Flavin-dependent halogenases regioselectively introduce halide substituents into electron-rich substrates under mild reaction conditions. FDHs depend on reduced flavin adenine dinucleotide (FADH2) as a cofactor, which is bound by a dedicated subdomain. As a first reaction step, FAD-C4a-OOH is formed, which subsequently oxidizes the halide ion, resulting in the formation of hypohalous acid (HOX). While BrvH preferentially brominated screening substrates, the X. campestris (Xcc) halogenases exclusively brominated them.

Xcc4156 and BrvH have short loops in both positions, resulting in a more open substrate-binding site compared with Trp halogenases and a solvent-accessible catalytic lysine residue. Like BrvH, Xcc4156 does not halogenate free tryptophan; these enzymes do, however, show activity towards free indole and indole derivatives. This can be explained by the lack of stabilization of tryptophan in the substrate-binding site. The FAD-binding loop (amino acids 47–56) of Xcc4156 does not have continuous electron density in chain B. Indeed, the loop is partly disordered in one chain of the apo structure and is fixed in an open conformation in the other chain. The FAD-binding loop, which changes its conformation between the apo and the FAD-bound form in related enzymes, is involved in a crystal contact in the apo Xcc4156 crystals. In apo Xcc4156, this site (Thr346 and Asn347) does not contain any bound halide. The asparagine in Xcc4156 is particularly interesting as its side chain occupies the position that would be taken up by the ribityl moiety of FAD in a FAD-bound halogenase, thus possibly hampering FAD binding. Thus, apo Xcc4156 crystals provide functional insight into FAD and bromide binding, even though neither the cofactor nor the halide is visible in the structure.

>[2x]GAMGHAPAPSESQRLVRRVVIAGGGTAGWMAAAALSKLLGRQLQITLVESDEIGTVGVGEATIPSLVTFHRLLEIDEAQFMAATQATFKVGIAFEHWRDVDRHYIHSFGHTGTDHWSAGFQHFWLKAHARGVARDFGDYCLELRAAQEGRFAHLPNGGMNYAYHLDAGLYARFLRRFSEGFGVQRIEGRIGSVQTDAHSGDIAALVLDDGTRIEGDLFLDCTGFRALLIGQTLGVGSEDWSRWLFADSALAVQTESVGAPVTFTRARADRAGWMWRIPLQHRVGNGIVYSSRYTDQDSAAQVLEHNLQGRALTTPRALRFTPNQRHRVWEKNCVALGLASGFLEPIESTNIHLIQRGIVRLLQTFPQVIDPVDIAEYNRQAAEEIAHIRDFVILHYHATDRRDTAFWRDCASMEIPDSLRHRMELFRQSGRVFHQGNELFAENSWIQVMLGQGIVPRHHHPVADLMGDAELSQFLEGIRQRVEATLARLPPHAEFLRRYCPAPAPPAPMPQPAPGTPLAAPAA> MFEQRVNSDVLTVSTVNSQDQVTQKPLRDSVKQALKNYFAQLNGQDVNDLYE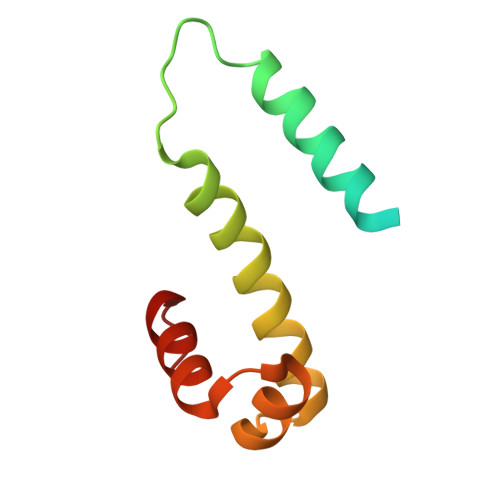LVLAEVEQALLDMVMQYTRGNQTRAALMMGINRGTLRKKLKKYGMN>MEPIIRIRNLHKWFGPLHVLKGIHLEVAPGEKLVIIGPSGSGKSTLIRTINRLEDFQEGEVVVDGLSVKDDRALREIRREVGMVFQQFNLFPHMTVLENVTLAPMRVRRWPREKAEKKALELLERVGILDQARKYPAQLSGGQQQRVAIARALAMEPKIMLFDEPTSALDPEMVGEVLDVMRDLAQGGMTMVVVTHEMGFAREVADRVVFMDGGQIVEEGRPEEIFTRPKEERTRSFLQRVLH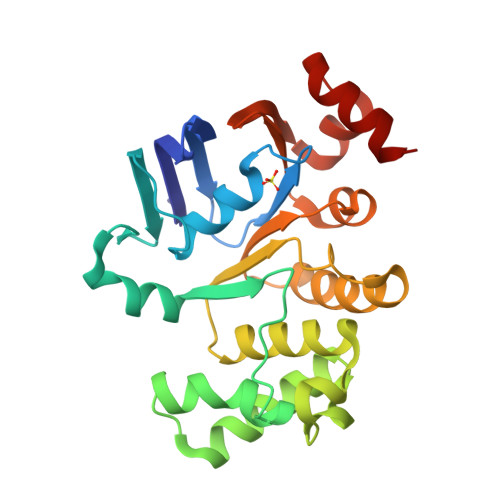H[4x]ZnT8, one of the 10 ZnTs that have been identified so far, is localized in the insulin secretory granules of pancreatic β cells and responsible for the accumulation of high level of zinc inside granules, which is required for the packing of insulin in the hexameric form. ZnT8 functions as a Zn2+/H+ exchanger. The structure of HsZnT8 in the outward-facing state shows a ‘V’-shaped dimeric architecture similar to the crystal structure of EcYiiP, with the two TMDs forming the branches, whereas the two tightly packed CTDs located at the base of the ‘V’ and mediating the majority of the dimerization interactions. Our structural and functional analyses reveal a total of 4 Zn2+ binding sites in each subunit, including one primary site in the TMD (STM), one site at the interface between TMD and CTD (SIF), and two adjacent sites located in an open pocket of CTD covered by a HCH motif from the N-terminal segment of neighboring subunit (SCD1 and SCD2).

Volta phase plate was employed in data collection to enhance the contrast for better image alignment, and the initial data was collected using the wild-type HsZnT8 (HsZnT8-WT) sample prepared in the presence of Zn2+ (1 mM). The single particle reconstruction yielded a map of the transporter in an outward-facing conformation, but the overall resolution of 4.1 Å is insufficient for accurate model building. From the structure of HsZnT8-WT determined in the presence of Zn2+, we also observed cryo-EM density from a third Zn2+ ion coordinated by His137 and His345 at the interface between CTD and TMD, which is designated as SIF. Interestingly, SIF is positioned right at the cytosolic entrance to the Zn2+ transport pathway and mutation of the two SIF histidines resulted in marked reduction in Zn2+ transport rate. As the physiological function of ZnT8 is to transport Zn2+ ions from low concentration cytosol (free Zn2+ concentration:~1 nM) to high concentration granule (free Zn2+ concentration:~120 nM), we suspect SIF can help trap Zn2+ ions and effectively increase the local Zn2+ concentration, which in turn facilitate the ion transport against over 100-fold concentration gradient. STM is surrounded by His106, Asp110, His220 and Asp224 at the middle of the membrane and exposed to the luminal solution in the outward-facing structure. The density of a bound Zn2+ can be defined in the EM map of HsZnT8-WT. Although the side-chains of those ligand residues are not well defined in the map due to the resolution limit, their locations and conservation likely point to a classical tetrahedral coordination as observed in EcYiiP structure. In the outward-facing conformation, TMs 1–5 are tightly bundled at the cytosolic half of TMD, occluding the space between STM and the cytosol; at the luminal half of TMD, TMs 2–6 enclose a deep cavity, penetrating into the central STM where Zn2+ binds and providing a solvent accessible passageway from luminal side.

>MYHCHSGSKPTEKGANEYAYAKWKLCSASAICFIFMIAEVVGGHIAGSLAVVTDAAHLLIDLTSFLLSLFSLWLSSKPPSKRLTFGWHRAEILGALLSILCIWVVTGVLVYLACERLLYPDYQIQATVMIIVSSCAVAANIVLTVVLHQRCLGHNHKEVQANASVRAAFVHALGDLFQSISVLISALIIYFKPEYKIADPICTFIFSILVLASTITILKDFSILLMEGVPKSLNYSGVKELILAVDGVLSVHSLHIWSLTMNQVILSAHVATAASRDSQVVRREIAKALSKSFTMHSLTIQMESPVDQDPDCLFCEDPCD[2x]>MGIMELARIDLSRDDLDKRIGGGIPHGSLIIIEGEESTGKSVLCQRLAYGFLQNRYSVTYVSTQLTTLEFIKQMNSLNYSINKKLLSGALLYIPVYPLIADNKKKDGFLKKVMETRAFYEKDVIIFDSISAL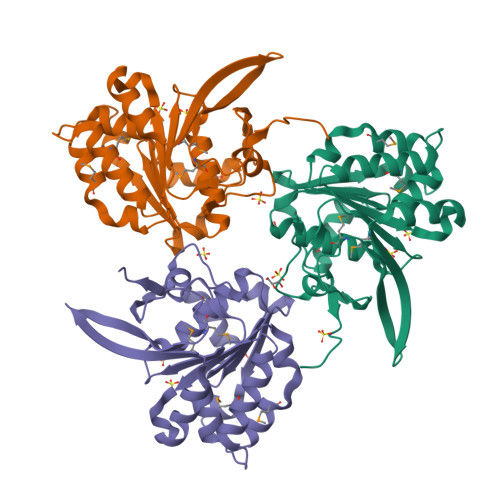IANDASEVNVDDLMAFFKRITALKKIIICTVNPKELPESVLTIIRTSATMLIRTELFTFGGDLKNLAKILKYNMAPGSYQKNIVFRVEPKIGIAVEIASVA[3x]>[12x]MCFSPKIKTPKMDTNQIRAVEPAPLTQEVSSVEFGGSSDETDTEGTEVSGRKGLKVERDDSVAKSKASGNGSARMKSSIRKSAFGGKK;>MGKKVKKAVKKVTKSVKKVVKEGARPVKQVAGGLAGLAGGTGEAQMVEVPQAAAQIVDVPEKEVSTEDEAQTESGRKKARAGGKKSLSVARSSGGGINI[6x];>[18x]MANVIKTVLTYQLDGSNRDFNIPFEYLARKFVVVTLIGVDRKVLTINTDYRFATRTTISLTKAWGPADGYTTIELRRVTSTTDRLVDFTDGSILRAYDLNVAQIQTMHVAEEARDLTTDTIGVNNDGHLDARGRRIVNLANAVDDRDAVPFGQLKTMNQNSWQARNEALQFRNEAETFRNQAEGFKNESSTNATNTKQWRDETKGFRDEAKRFKNTAGQYATSAGNSASAAHQSEVNAENSATASANSAHLAEQQADRAEREADKLENYNGLAGAIDKVDGTNVYWKGNIHANGRLYMTTNGFDCGQYQQFFGGVTNRYSVMEWGDENGWLMYVQRREWTTAIGGNIQLVVNGQIITQGGAMTGQLKLQNGHVLQLESASDKAHYILSKDGNRNNWYIGRGSDNNNDCTFHSYVHGTTLTLKQDYAVVNKHFHVGQAVVATDGNIQGTKWGGKWLDAYLRDSFVAKSKAWTQVWSGSAGGGVSVTVSQDLRFRNIWIKCANNSWNFFRTGPDGIYFIASDGGWLRFQIHSNGLGFKNIADSRSVPNAIMVENE;>MALISQSIKNLKGGISQQPDILRYPDQGSRQVNGWSSETEGLQKRPPLVFLNTLGDNGALGQAPYIHLINRDEHEQYYAVFTGSGIRVFDLSGNEKQVRYPNGSNYIKTANPRNDLRMVTVADYTFIVNRNVVAQKNTKSVNLPNYNPNQDGLINVRGGQYGRELIVHINGKDVAKYKIPDGSQPEHVNNTDAQWLAEELAKQMRTNLSDWTVNVGQGFIHVTAPSGQQIDSFTTKDGYADQLINPVTHYAQSFSKLPPNAPNGYMVKIVGDASKSADQYYVRYDAERKVWTETLGWNTEDQVLWETMPHALVRAADGNFDFKWLEWSPKSCGDVDTNPWPSFVGSSINDVFFFRNRLGFLSGENIILSRTAKYFNFYPASIANLSDDDPIDVAVSTNRIAILKYAVPFSEELLIWSDEAQFVLTASGTLTSKSVELNLTTQFDVQDRARPFGIGRNVYFASPRSSFTSIHRYYAVQDVSSVKNAEDITSHVPNYIPNGVFSICGSGTENFCSVLSH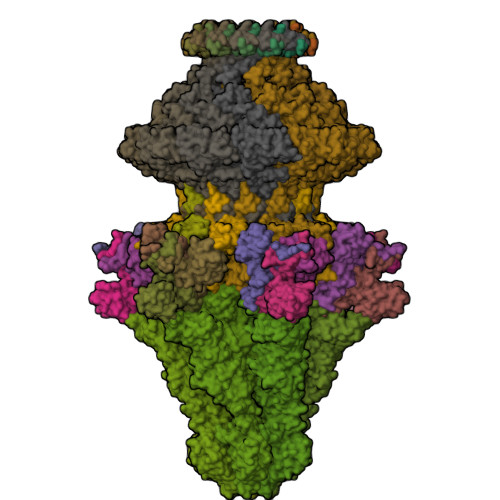GDPSKIFMYKFLYLNEELRQQSWSHWDFGENVQVLACQSISSDMYVILRNEFNTFLARISFTKNAIDLQGEPYRAFMDMKIRYTIPSGTYNDDTFTTSIHIPTIYGANFGRGKITVLEPDGKITVFEQPTAGWNSDPWLRLSGNLEGRMVYIGFNINFVYEFSKFLIKQTADDGSTSTEDIGRLQLRRAWVNYENSGTFDIYVENQSSNWKYTMAGARLGSNTLRAGRLNLGTGQYRFPVVGNAKFNTVYILSDETTPLNIIGCGWEGNYLRRSSGI[6x];>[12x]MRSYDMNVETAAELSAVNDILASIGEPPVSTLEGDANADAANARRILNKINRQIQSRGWTFNIEEGITLLPDVYSNLIVYSDDYLSLMSTSGQSIYVNRGGYVYDRTSQSDRFDSGITVNIIRLRDYDEMPECFRYWIVTKASRQFNNRFFGAPEVEGVLQEEEDEARRLCMEYEMDYGGYNMLDGDAFTSGLLTR;>[12x]MAEKRTGLAEDGAKSVYERLKNDRAPYETRAQNCAQYTIPSLFPKDSDNASTDYQTPWQAVGARGLNNLASKLMLALFPMQTWMRLTISEYEAKQLLSDPDGLAKVDEGLSMVERIIMNYIESNSYRVTLFEALKQLVVAGNVLLYLPEPEGSNYNPMKLYRLSSYVVQRDAFGNVLQMVTRDQIAFGALPEDIRKAVEGQGGEKKADETIDVYTHIYLDEDSGEYLRYEEVEGMEVQGSDGTYPKEACPYIPIRMVRLDGESYGRSYIEEYLGDLRSLENLQEAIVKMSMISSKVIGLVNPAGITQPRRLTKAQTGDFVTGRPEDISFLQLEKQADFTVAKAVSDAIEARLSFAFMLNSAVQRTGERVTAEEIRYVASELEDTLGGVYSILSQELQLPLVRVLLKQLQATQQIPELPKEAVEPTISTGLEAIGRGQDLDKLERCVTAWAALAPMRDDPDINLAMIKLRIANAIGIDTSGILLTEEQKQQKMAQQSMQMGMDNGAAALAQGMAAQATASPEAMAAAADSVGLQPGI>MPGSIPLIGERFPEMEVTTDHGVIKLPDHYVSQGKWFVLFSHPADFTPVSTTEFVSFARRYEDFQRLGVDLIGLSVDSVCSHIKWKEWIERHIGVRIPFPIIADPQGTVARRLGLLHAESATHTVRGVFIVDARGVIRTMLYYPMELGRLVDEILRIVKALKLGDSLKRAVPADWPNNEIIGEGLIVPPPTTEDQARARMESGQYRSLDWWFSWDTPASRDDVEEARRY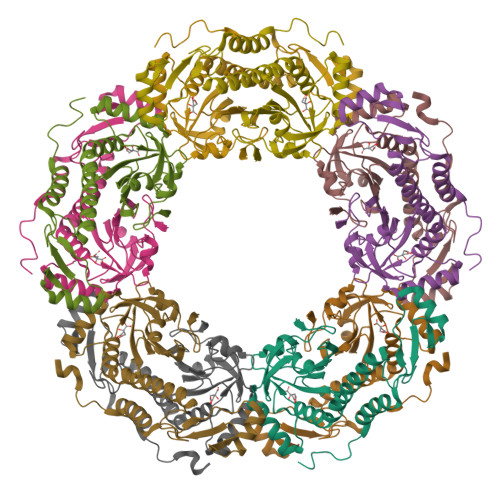LRRAAEKPAKLLYEEARTHLH[10x]> MTLELQLKHYITNLFNLPKDEKWECESIEEIADDILPDQYVRLGALSNKILQTYTYYSDTLHESNIYPFILYYQKQLIAIGYIDENHDMDFLYL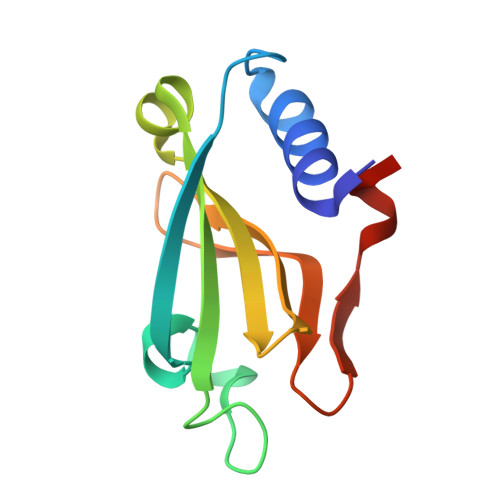HNTIMPLLDQRYLLTGGQ>[3x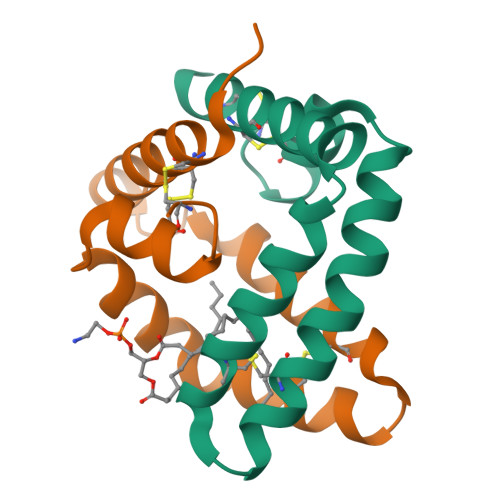]MDGDVCQDCIQMVTDIQTAVRTNSTFVQALVEHVKEECDRLGPGMADICKNYISQYSEIAIQMMMHMQPKEICALVGFCDE>GSHMDQDSLSSSLKTCYKYLNQTSRSFAAVIQALDGEMRNAVCIFYLVLRALDTLEDDMTISVEKKVPLLHNFHSFLYQPDWRFMESKEKDRQVLEDFPTISLEFRNLAEKYQTVIADICRRMGIGMAEFLDKHVTSEQEWDKYCHYVAGLVGIGLSRLFSASEFEDPLVGEDTERANSMGLFLQKTNIIRDYLEDQQGGREFWPQEVWSRYVKKLGDFAKPENIDLAVQCLNELITNALHHIPDVITYLSRLRNQSVFNFCAIPQVMAIATLAACYNNQQVFKGAVKIRKGQAVTLMM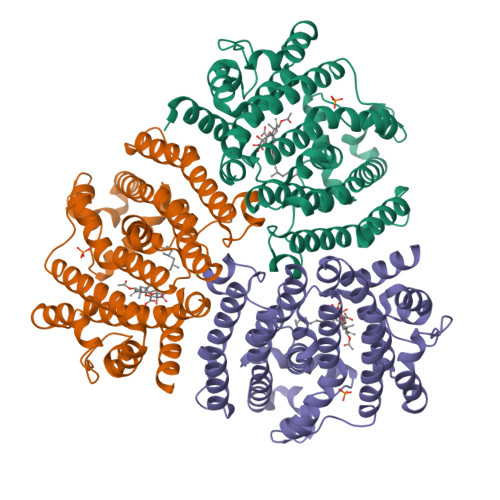DATNMPAVKAIIYQYMEEIYHRIPDSDPSSSKTRQIISTIRTQN[6x]> THWFHRNPLKATAPVSFNYYGVVTGPSASKICNDLRSSRARLLELFTDLSCNPEMMKNAADSYFSLLQGFINSLDESTQESKLRYIQNFKWTDTLQGQVPSAQQDA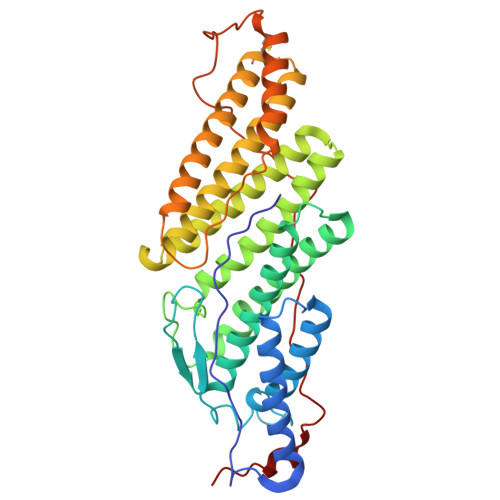VFELISMGFNVALWYTKYASRLAGKENITEDEAKEVHRSLKIAAGIFKHLKESHLPKLITPAEKGRDLESRLIEAYVIQCQAEAQEVTIARAIELKHAPGLIAALAYETANFYQKADHTLSSLEPAYSAKWRKYLHLKMCFYTAYAYCYHGETLLASDKCGEAIRSLQEAEKLYAKAEALCKEYGETKGPGPTVKPSGHLFFRKLGNLVKNTLEKCQRENGFIYFQKIPTEAPQLELKANYGLVEPIPFEFPPTSVQWTPETLAAFDLTK>MTSTNPVKDSYNKDAVFTYELIANPDADYSDQKLILKKEISYIKLNLGINQDNKNAPSYIFNLLDDNVYYGFYRDTQDMNRIENKYTYAFKKEAENFDNLQKFNATYEGQFWFSSIDTPNVPTVARAFLTYNNGRVDGEILAKHWNEKLFQITGFDNNPRKVEIFPTVEYLPNSGTRLTKGATSPHRFQMDLHFINSTNGEKNKYLVGQGSTEQYWGVLGMAAAQELALVPRGSSAHHHHHHHHHH[2x]

Here, we report that PmSLP binds host complement factor I (FI) and facilitates cleavage of complement components C3b and C4b independently of any cofactors (e.g., FH, C4BP), thereby allowing the pathogen to evade host defence. We show that PmSLP-1 not only exhibits a high-affinity interaction with bovine complement factor I, but it also serves as a co-factor for factor I to promote cleavage of complement C3b and C4b. This protein-protein interaction thus plays a crucial role in modulating the complement activation on the bacterial cell surface and increasing bacterial resistance to complement-mediated killing.

To identify structural features of PmSLP-1 that would aid in its function, we sought a high-resolution crystal structure of the protein. Thus, to improve the chance of protein crystallization, we modified the protein construct by removing the first 94 N-terminal residues, predicted to be disordered, and mutating a stretch of surface-exposed, charged residues (E315A, K316A, and K317A) at the C-terminus. By removing the flexible N-terminal region and lowering the surface entropy on the C-terminus, we were able obtain protein crystals with high diffraction quality. The modified variant PmSLP-195 and its selenomethionine derivative were then used to solve and refine the protein structure to a resolution of 2.0 Å. PmSLP-1 is a predominantly β-stranded structure which forms an N-terminal domain (NTD) and a C-terminal domain (CTD) connected by a 13-residue linker peptide. The eight β-strands on the C-terminus fold into a barrel, coined the barrel domain, and the six β-strands on the N-terminus form an open-hand-like structure, referred to as the handle domain. These two domains are held stably together through a network of hydrogen bonds. We also observed two short helices present in the loop regions of the protein. Noticeably, the overall architecture of PmSLP-1 resembles that of previously known Slam-dependent SLPs. We postulate that the conserved β-barrel CTD serves as a Slam-recognition motif whereas the varying NTD and loop regions dictate the protein function through specific protein interactions.> ETDEEPEEPGRRGSFVEMVDNLRGKSGQGYYVEMTVGSPPQTLNILVDTGSSNFAVGAAPHPFLHRYYQRQLSSTYRDLRKGVYVPYTQGKWEGELGTDLVSIPHGPNVTVRANIAAITESDKFFINGSNWEGILGLAYAEIARPDDSLEPFFDSLVKQTHVPNLFSLQLCGAGFPLNQSEVLASVGGSMIIGGIDHSLYTGSLWYTPIRREWYYEVIIVRVEIN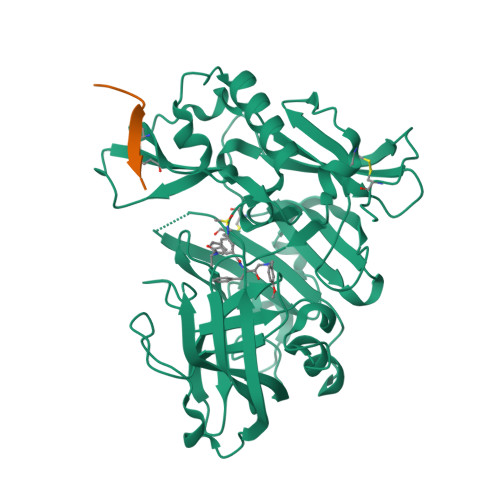GQDLKMDCKEYNYDKSIVDSGTTNLRLPKKVFEAAVASIKAASSTEKFPDGFWLGEQLVCWQAGTTPWNIFPVISLYLMGEVTNQSFRITILPQQYLRPVEDVATSQDDCYKFAISQSSTGTVMGAVIMEGFYVVFDRARKRIGFAVSACHVHDEFRTAAVEGPFVTLDMEDCGYNIPQTDEST;> XALYPYFLPISAK>HPETLVKVKDAEDQLGARVGYIELDLNSGKILESFRPEERFPMMSTFKVLLCGAVLSRVDAGQEQLGRRIHYSQNDLVEYSPVTEKHLTDGMTVRELCSAAITMSDNTAANL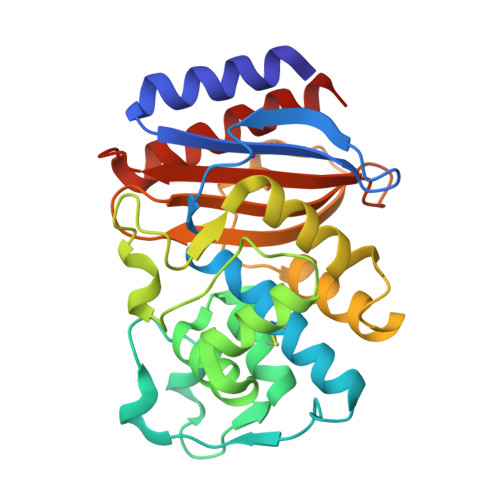LLTTIGGPKELTAFLHNMGDHVTRLDRWEPELNEAIPNDERDTTTPAAMATTLRKLLTGELLTLASRQQLIDWMEADKVAGPLLRSALPAGWFIADKSGAGERGSRGIIAALGPDGKPSRIVVNYTTGSQATMDERNRQIAEIGASLIKHW[4x]>SMGEIESYCNKELGPLPTKAPTLSKNVLDLFSLKGKVASVTGSSGGIGWAVAEAYAQAGADVAIWYNSHPADEKAEHLQKTYGVRSKAYKCNISDPKSVEETIS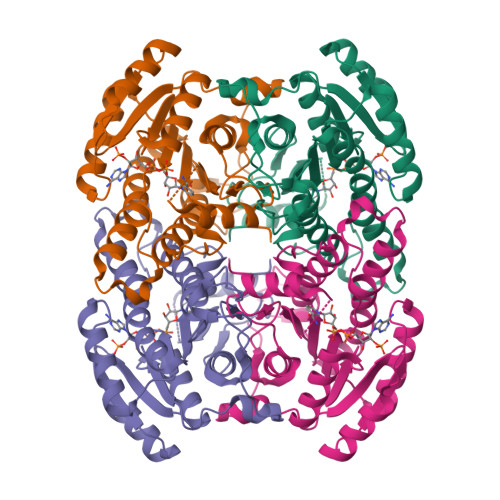QQEKDFGTIDVFVANAGVPWTEGPEINVDNYDSWNKIINLDLNGVYYCAHTVGKIFKKNGKGSLVITSSMSGTIVNVPQLQAAYNAAKAACTHLTKSLAVEWAPFARVNCVSPGYIATEISDFVEKDMKAKWWQLTPLGREGLAQELVGAYLYLASNASTYTTGANLAVDGGYTCP[2x]>VTAVPTDSAEKPAVADAGVRSVTRVIDLLELFDAAHPTRSLKELVEGTKLPKTTVVRLVATMCARSVLTSRADGSYSLGPEMLRWVRLAGRTWAPPEEVVDIMRQLSADTGETVNLYIRQGLSRVVVAQCESTATVRSVIPLGVPYPLWAGAAGKILLLAAPELIDDVAADSPH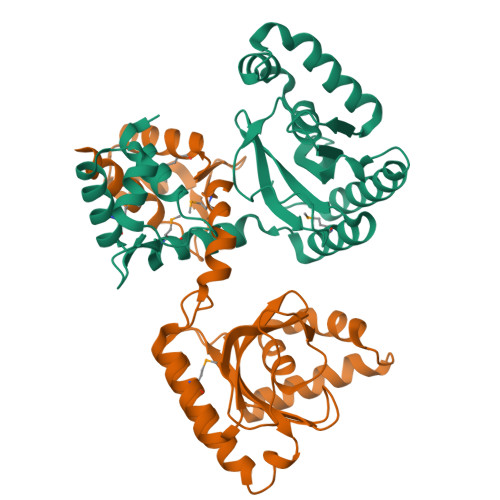GPEFADQLREKVEDGRERGYQLVHGERELGSSGLSFPLVDSHGTVVAALTLGGPTGRFTEDRTPHYIECTRAAAEEISAIGLPGLD[4x]>KMPTLLRVYIDG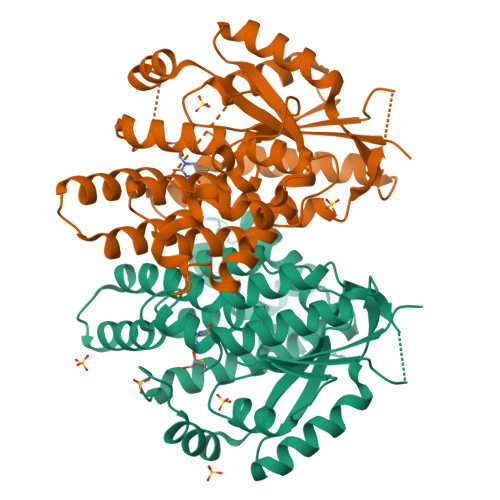PHGMGKTTTTQLLVALGSRDDIVYVPEPMTYWRVLGASETIANIYTTQHRLDQGEISAGDAAVVMTSAQITMGMPYAVTDAVLAPHIGGEAGSSHAPPPALTLIFDRHPIAALLCYPAARYLMGSMTPQAVLAFVALIPPTLPGTNIVLGALPEDRHIDRLAKRQRPGERLDLAMLAAIRRVYGLLANTVRYLQCGGSWREDWGQLSGTAVPPQGAEPQSNAGPRPHIGDTLFTLFRAPELLAPNGDLYNVFAWALDVLAKRLRSMHVFILDYDQSPAGCRDALLQLTSGMVQTHVTTPGSIPTICDLARTFAREMGEAN[2x]2-(acetylamino)-2-deoxy-1-O-[(S)-{[(R)-{[(2Z,6Z,10E,14E,18E)-3,7,11,15,19,23-hexamethyltetracosa-2,6,10,14,18,22-hexaen-1-yl]oxy}(hydroxy)phosphoryl]oxy}(hydroxy)phosphoryl]-alpha-D-glucopyranose 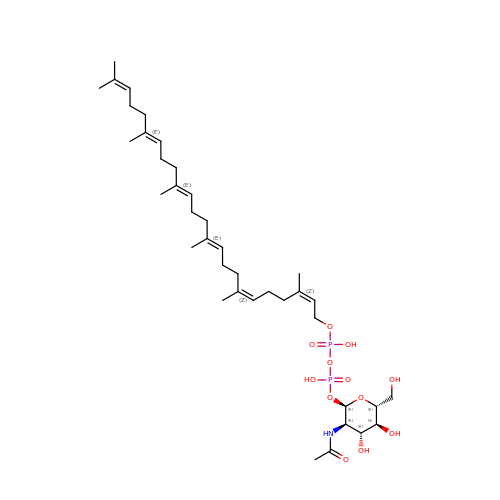| C38 H65 N O12 P2 | DOEXPFXURIPLFY-QTFKUDQZSA-N> SNAETVKCQRQETKSDREFAKLEDKYDANLGVFALDTGTNKTVTYHPDERFAYASTHKALAVGALLQQKSIEDLNERIFYTRDDLVNYNPITEKHVDTGMTLRELADASLRYSDNTAGNLILQQLDGPD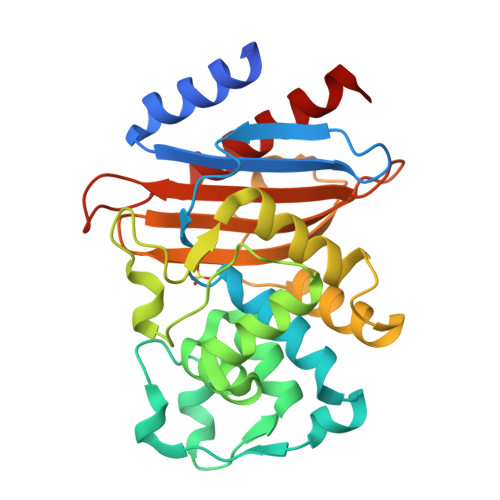GFKEALEKIGDNVTLPERFEPDLNEVNPGETHDTSTPRALAASLQKYVLGQALPEDKRALLTDWMKRNTTGDALIRAGVPKSWEVADKTGAGSYATRNDIAILWPPNGDPIVLAILSNRTEKDAEYNDKLIAEAAKQAVKTLKITRK MONO-TRANS, OCTA-CIS DECAPRENYL-PHOSPHATE 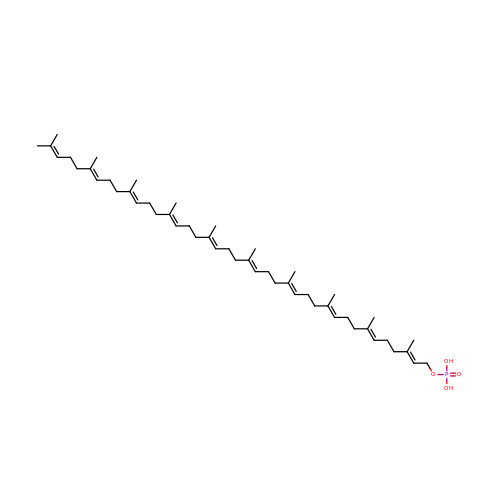| C50 H83 O4 P | XBEJBEIXLWRYBT-DJNGBRKISA-N> SGTFFKDYQKKNVMRLLQDSLEKIINEWLKTDDESHTKLKSLQELSEMDINATSFAEHSPLPDFVTRLWLDPHKALDAMDKNISKNEIRKLIKETAREIELVFTH;> SMTTSKLEKTGLHVHEKIKHMVKNYGTMITGIPAEILGQNEAEISVGYVKKM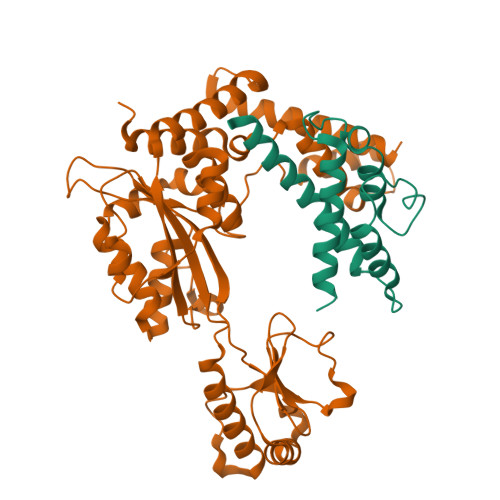GNMKENIAEVVRKSEMTQPTNSCGKASNEVCDLLLGTEGASEFEKSSYQVLSGDGSNLKGSLPNKNLLVRVEMDRFNAPQKYQKIKREEFNPETAEKNKIYLLEDQLVYLDIFGKVIDLGQTSDTCHRLFNAITTPFYQNYILYDEYIDPEESAEEAAMFEMGEIVKAKMKNIDCWTATHSFTIFVPESDSEDTRTLYPYQAYWTSHTLQQWFSGDKDEKLSRLGIDGYIEKLALLGTTTDSKIRSSIYGELFSPPGKEHVFCTGMNEKFSPLRVKFKVTEVNPEIALQNLEEVQEFIDTNYPGENAKDQCELYKIKAQEAMTKQLEMRLLIEP>[5x]MRLSYEALEWRTPIENSTEPVSLPPPPPFFGQERAREALELAIRGGFHAYLVGPPSLGKHEALLAYLSTQSVETPPDLLYVPLSERKVAVLTLPSGQEIHLAEAVEGLLLEVNRLDELFRQGSFLREKTQL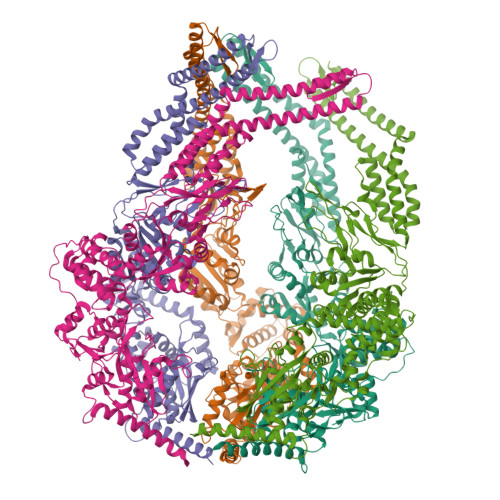EARFKEAREQQLEALRREAQEAGFALSTNGERLELTGPGPVPAELSARLEEVTLGSLAASAELEVALRRLRRDWALHYLNNRFEPLFQRFPQARAYLEALRARLARYAETGEPLDPAQWRPNLLTSSSSGTPPPIVYEPYATAPRLFGRLDYLVDRGVWSTNVSLIRPGAVHRAQGGYLILDALSLKREGTWEAFKRALRNGQVEPVTEPQAPAGLEVEPFPIQMQVILVGTPEAFEGLEEDPAFSELFRIRAEFSPTLPASPENCTALGGWLLAQGFQLTQGGLTRLYDEARRMAEQRDRMDARLVEIRALAEEAAVLGGGLLTAESVEQAIAAREHRSFLSEEEFLRAVQEGVIRLRTTGRAVGEVNSLVVVEAAPYWGRPARLTARAAPGRDHLISIDREAGLGGQIFHKAVLTLAGYLRSRYIEHGSLPVTISLAFEQNYVSIEGDSAGLAELVAALSAIGNLPLRQDLAVTGAVDQTGKVLAVGAINAKVEGFFRVCKALGLSGTQGVILPEANLANLTLRAEVLEAVRAGQFHIYAVETAEQALEILAGARMEGFRGLQEKIRAGLEAFARLEEGHDKEDREKLAAALEHHHHHH5-amino-N-hydroxypentanamide | C5 H12 N2 O2 | 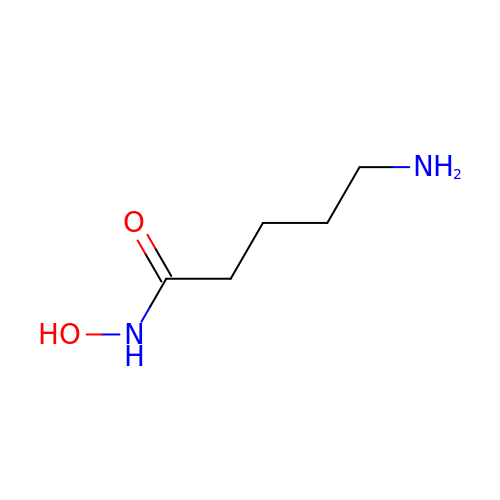YEOWNCJWBHIJNK-UHFFFAOYSA-N>[4x]SMPPPPEVSPVTGNPVSPHYIHSSTLHFQDVNGRSLVLRGVNLSGSAKHPNNQPSHIREGFWETAEAGKGDFINKPLNLDDGSADLHLARLKAWGYNLLRYVFTWESLEHAGPKEYDYAYMDYIIAVLRKCKEWGFRVFMDPHQDVWSRFTGGSGAPLWTLYACGIDPYHLTATAAAYLHCEWPSAESPKPQDFPAMIWGTNYTHLANQTIWTFFFAGKTYAPKCIIDGKNIQDFLQDHFIDAVGELAKRIAEEAGDLLDECVIGWDSINEPGEGLIGCKDLAVIPAEQQLKKGPSPTPIEGMRLGMGEAQDVQAWNFGPMGPYRGSRQTIDPKGVKLWLSKEDDVKRGSGKWGWTRGKEWALGTCIWAHHGVWEIATSTLLRPDYFSTLPTNPGHQVDFVDDFWALHWLAYSSRIRLHHPESIHFIQAPVLR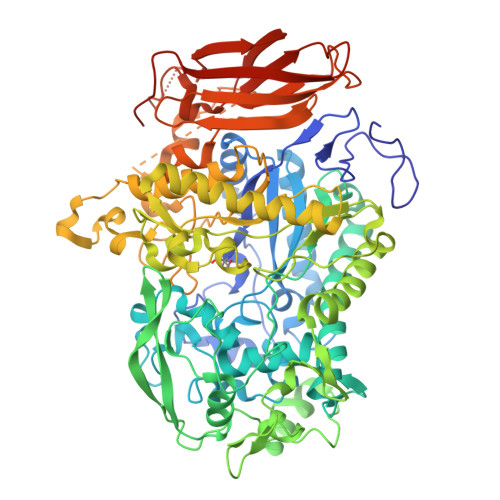QPPKLPESFLKGRACSSPHFYDGLTLMTKHWNWFNADAIGVIRKKYWSIVQAVRIGEGPIRKMIQGELAVLKQDTIDILGNYPTLVGEIGIPYDMDDKKAYGYVDGGRGEGDYSSQQKAMDCSMNACDGPNCLNYAIWNYVPDNVHEWGDNWNGEDLSLWSVDDKEQESYHDSPRSDTPNFSTNSNSLTNSSATLTVPMSGASKLRPSPSVIDSGDFSPTLILDGSRAVAAFCRPYPVATVGIPERIDFDITSTKFKYAVRVRADDIANEQVYTEIYLPFVHYAASLNASYSSFAQLSLDVTIVASHGRVEIQGQTLRWWYPVPGTGEEVYTIEVQRNGGALRRDLGYVQQGNFLDVCPECVIA7-[(3-aminopropyl)amino]-1-methoxyheptane-2,2-diol 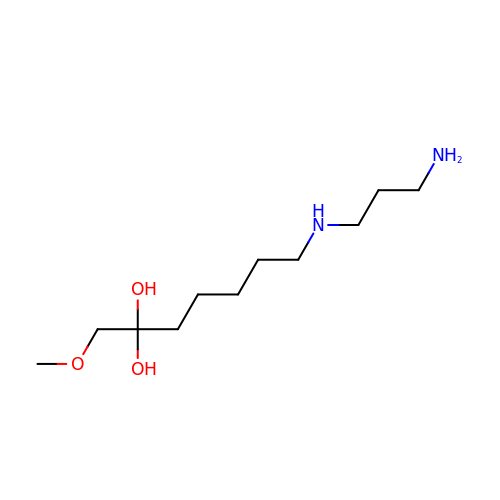| C11 H26 N2 O3 | ATZSVPANUKMESL-UHFFFAOYSA-N>MTTTNEIRVAEVADAGVVAKLLRDFNTEFDTPVPEGLEERFAQIIAHDDAFVLLAGDIGFAYVTLRPSPYYDGPVAMLDELYVAPAHRNRGVGTALLQRVFEEIRKHSAGELQINVDEVDTDARRFYERH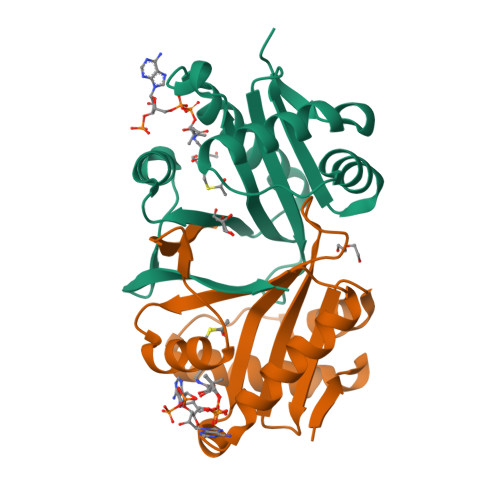GLTNIEQGSRMLLYIREL[2x]> MNGYDPVLLSRILTELTLTVHIIYATIGVGVPLMIAIAQWVGIRKNDMHYILLARRWTRGFVITVAVGVVTGTAIGLQLSLLWPNFMQLAGQVISLPLFMETFAFFFEAIFLGIYLYTWDRFENQKKHLLLLIPVAIGSSASAMFITMVNAFMNTPQGFELKNGELVNI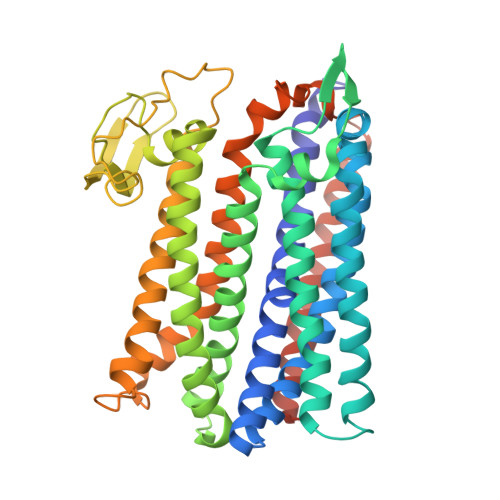DPIVAMFNPAMPTKVAHVLATSYMTSAFVLASIAAWHLWKGNRHIYHRKALHLTMKTAFIFSVASALVGDLSGKFLAEYQPEKLAAAEWHFETSSHAPLILFGTLEEDNEVKYALEIPYALSILAHNHPAAVVTGLNDIPEDERPPLYIHYLFDVMVTIGVFLMVVAAVYWLGSIFRWKWTAKNWFFGLLVAGGPLAMIAIEAGWYLAEVGRQPWILRGYMKTAEGATTSAHVDTMLVLFCLLYIVLVIASATVLIRMFRRNPVERELEERANRGEVAP>[2x]MNEEKREELLEEAKRLLEESLKLLKQAYNTPIEIDLPISGGVKAILYNGKVYLIYENGKVEEIEIPEDDILYPIYNKYIETLKEALKTVEKLQEELEE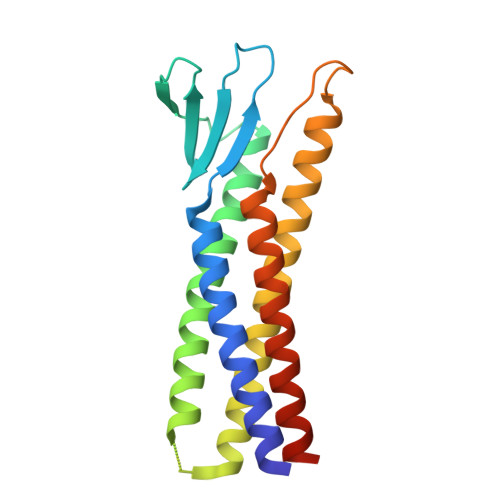LLENEEDGELSEEERLEKLKELAEELKETAEKLLKSIEEFSKFLEELKKKLPKNIKLNINYSSINLAKEAAEKALEASELLEEVYESSGSGHHHHHH2,3-dichlorophenol 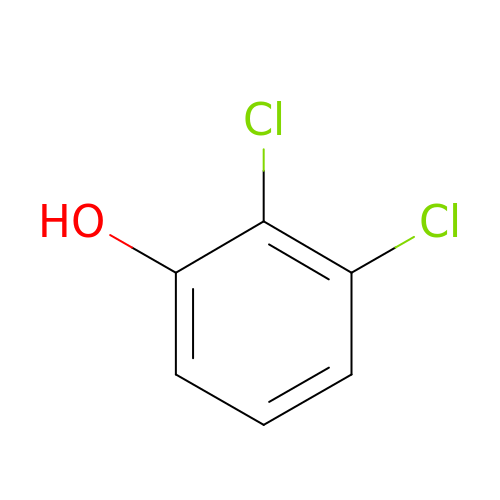| C6 H4 Cl2 O | UMPSXRYVXUPCOS-UHFFFAOYSA-N>[4x]MKKLFLVFWWHMHQPLYREPYTGEYLLPWTFFHAVKDYYDMPAYLKDFEIKLNFNLTPVLIDQIQEYAQGKAKDVFLEAIRKDPDDLEKEEVEKLIEFTKLNYEKPIYRFERIRELMNKEKLNREELLDLQTLNLLAWCGRTLRKDLKDLLNKGRNYTQEEKEYVLNKYFEIIKKTLSIYREIKEEGKGSVSTSPYYHPL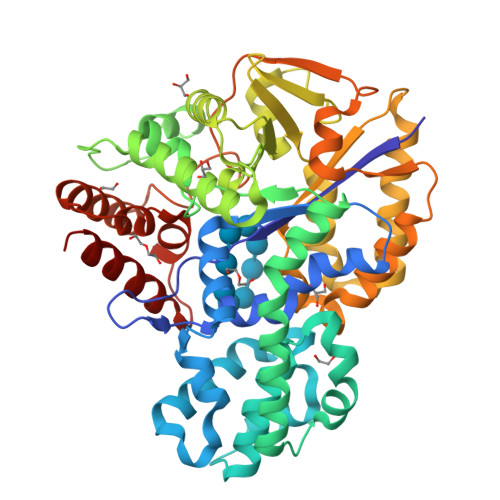IPILLNPNCVYETTPNVKIPDFAVSFREDASKHVELAKEKYFEIFGEHPVYMWPPEASVSNEALELYYEKGINMLATDEVILKNSVERASPYLRYYFRELISVFFRDKTLSDLIGFSYHAWNAEDAVRDFIGRLKKIHESVDFQPVVFVVLNGENCWEYYEENGIPFLEKLYSTLEKEEWIETLTLEEAMRKEDVKTEVIESVKAGTWFDGNFLKWIGNKEKNEYWKILIEAKKKAKNDYILVAEGSDWFWWQGEEKAPFVEVFDKLFRSFVRRAQE>[4x]GPGSMKKELRVGVLISGRGSNLEALAKAFSTEESSVVISCVISNNAEARGLLIAQSYGIPTFVVKRKPLDIEHISTVLREHDVDLVCLAGFMSILPEKFVTDWHHKIINIHPSL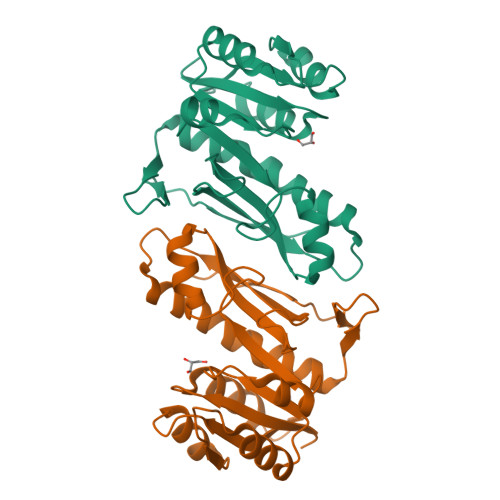LPSFKGLNAQEQAYKAGVKIAGCTLHYVYQELDAGPIIMQAAVPVLREDTAESLASRILAAEHVCYPKGVKLIAQDKIKLCDDGTVQCTGEDELFLFQENF> HMGRSQNSEFETASDEPIAVIGLSCRLPKASGPQELWQLLDDGASAVTRVPADRETPPSTEEESADGEAAGARWGGFLDRVDTFDAGFFGISPREAAAMDPQQRLVLELSWEALEGAGLVPATLRDTGLGVFVGAARDDYATLYRRREGRAVDHHAMTGLHRSLIANRISYALGAHGPSMVVDTGCSSSLVAVHLACESLRRGESDIALAGGVNLNIAAESARETAAFGGLSPDGQCFTFDARANGFVRGEGGGLVVLKTLRRALADGDLVHGVILASAVNNDGPSDTLTTPSRRAQESLLTRVYRRAGVTPTEVGYVELHGTGTKVGDPIEAAALGAVLGTGRDTPLPVGSIKTNIGHLEGAAGIAGLIKALLQLRRRRLVPSLNFSTPNPDIPLDALNLRVQQESAPWATPSGGGRTLVAGVSSFGMGGTNCHVVVSAAPVPEDGETTSEAGATGPDSGPALLPWVVSARSPQALRDQAGRLAAWADSPAGREASPVDIGWSLATSRTHFEYRAVVSGSDRDELVASLRALASGSPVTAAGAVDGGGRLGLVFSGQGSQRAGMGREL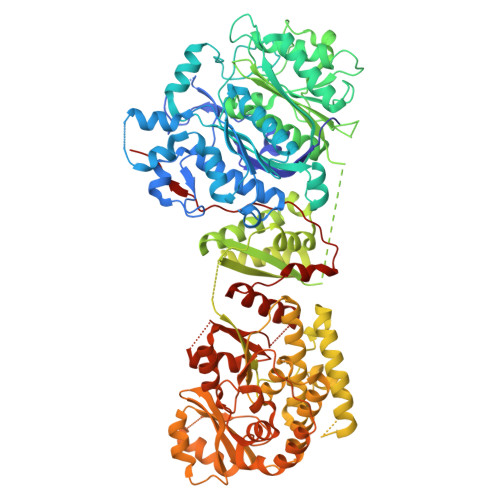YVAFPVFAEAFDEVCGVLDEVMGALPPSEGWAGSLREVMFEVSSDLLDETGFTQPALFAFEVALYRLLESWGVAGEVVAGHSVGEIAAVHVAGVLSLADACALVAARGRLMQGLPSGGAMVAVEASEEEVTALLAGREGEVGIGAVNGPRSVVVSGGVAVVEEVAAHFAGLGRRARRLKVSHAFHSPLMDPMLEDFGRVVAGLSFAVPELTVVSGLTGAVVSADELCSVGYWVRHAREAVRFADAVGAMAGVGVGRFVEVGPGGVLSALVRECLAEGGAGSVVAAVRGNRAEPVALLSAVGELFADGYPVDWTAYFAGWPAARVELPTYAFQRSRHWLENVPELAVS> MSNAALATAPHALELDVHPVAGRIGAEIRGVKLSPDLDAATVEAIQAALVRHKVIFFRGQTHLDDQSQEGFAKLLGEPVAHPTVPVVDGTRYLLQLDGAQGQRANSWHTDVTFVEAYPKASILRSVVAPASGGDTVWANTAAAYQELPEPLRELADKLWAVHSNRYDYASLKPDIDPAKLERHRKVFTSTVYETEHPVVRVHPISGERALQLGHFVKRIKGYSLADSQHLFAVLQGHVTRLENTVRWRWEAGDVAIWDNRATQHYAVDDYGTQPRIVRRVTLAGEVPVGVDGQLSRTTRKG;>MSNAALATAPHALELDVHPVAGRIGAEIRGVKLSPDLDAATVEAIQAALVRHKVIFFRGQTHLDDQSQEGFAKLLGEPVAHPTVPVVDGTRYLLQLDGAQGQRANSWHTDVTFVEAYPKASILRSVVAPASGGDTVWANTAAAYQELPEPLRELADKLWAVHSNEYDYASLKPDIDPAKLERHRKVFTSTVYETEHPVVRVHPISGERALQLGHFVKRIKGYSLADSQHLFAVLQGHVTRLENTVRWRWEAGDVAIWDNRATQHYAVDDYGTQPRIVRRVTLAGEVPVGVDGQLSRTTRKG[2x];> MSNAALATAPHALELDVHPVAGRIGAEIRGVKLSPDLDAATVEAIQAALVRHKVIFFRGQTHLDDQSQEGFAKLLGEPVAHPTVPVVDGTRYLLQLDGAQGQRANSWHTDVTFVEAYPKASILRSVVAPASGGDTVWANTAAAYQELPEPLRELADKLWAVHSNEYDYASLKPDIDPAKLERHRKVFTSTVYETEHPVVRVHPISGERALQLGHFVKRIKGYSLADSQHLFAVLQGHVTRLENTVRWRWEAGDVAIWDNRATQHYAVDDYGTQPRI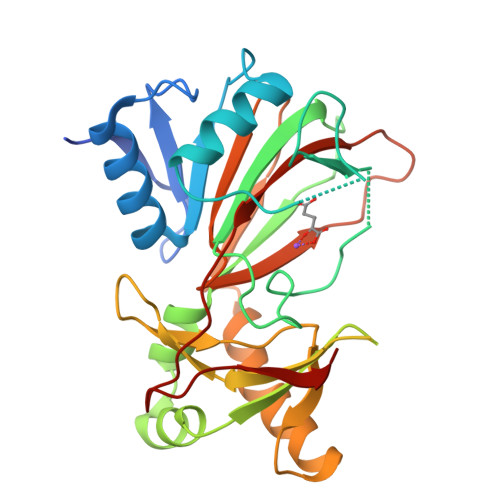VRRVTLAGEVPVGVDGYLSRTTRKG2-fluorophenol | C6 H5 F O | 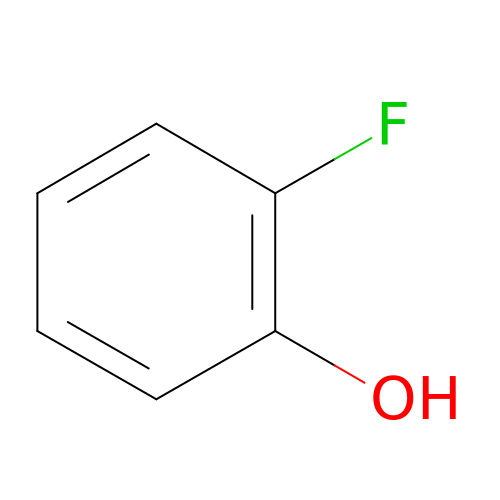HFHFGHLXUCOHLN-UHFFFAOYSA-N> MELKHSISDYTEAEFLQLVTTICNADTSSEEELAKLVTHFEEMTEHPSGSDLIYYPKEGDDDSPSGIVNTVKQWRAANGKSGFKQG;> MESKRNKPGKATGKGKPVGDKWLDDAGKDSGAPIPDRIADKLRDKEFKSFDDFRKAVWEEVSKDPELSKNLNPSNKSS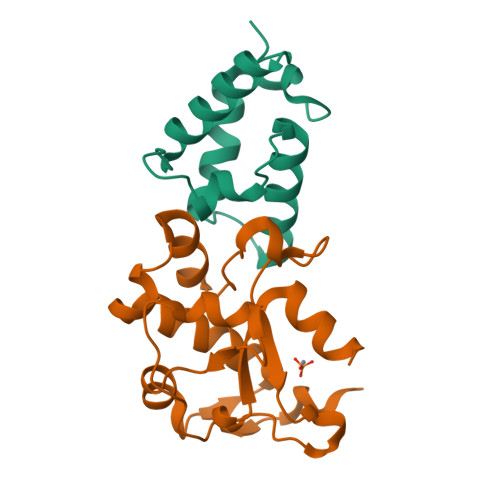VSKGYSPFTPKNQQVGGRKVYELHHDKPISQGGEVYDMDNIRVTTPKRHIDIHRGK> GSPCVEVVPNITYQCMELNFYKIPDNLPFSTKNLDLSWNPL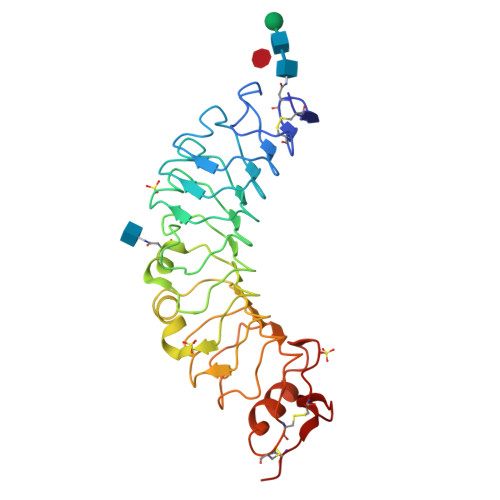RHLGSYSFFSFPELQVLDLSRCEIQTIEDGAYQSLSHLSTLILTGNPIQSLALGAFSGLSSLQKLVAVETNLASLENFPIGHLKTLKELNVAHNLIQSFKLPEYFSNLTNLEHLDLSSNKIQSIYCTDLRVLHQMPLLNLSLDLSLNPMNFIQPGAFKEIRLKELALDTNQLKSVPDGIFDRLTSLQKIWLHTNPWDCSCPRIDYLSRWLNKNSQKEQGSAKCSGSGKPVRSIICPT>[4x]MNAHSKEMAPLMGKRTTAPGGNPVVLTEKRPADLTPTKKSAHFFLEIEGFEPNPTVTKTSPPIFSKPMDSNIRQCLSGNCDDMDSPQSPQDDVTETPSNPNSPSANLAKEEQRQKKKRLKKRIFAAVSEGCVEELRELLQDLQDLCRRRRGLDVPDFLMHKLTASDTGKTCLMKALLNINPNTKEIVRILLAFAEENDILDRFINAEYTEEAYEGQTALNIAIERRQGDITAVLIAAGADVNAHA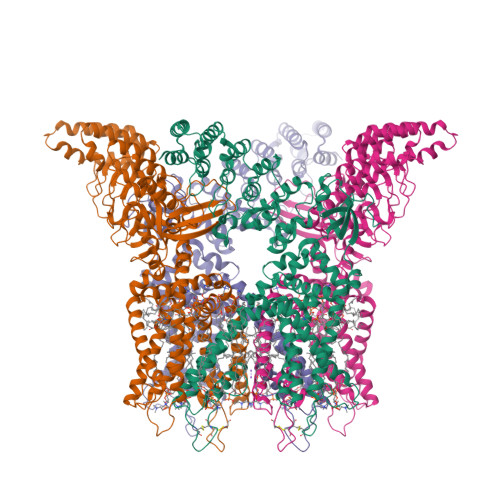KGVFFNPKYQHEGFYFGETPLALAACTNQPEIVQLLMENEQTDITSQDSRGNNILHALVTVAEDFKTQNDFVKRMYDMILLRSGNWELETMRNNDGLTPLQLAAKMGKAEILKYILSREIKEKPLRSLSRKFTDWAYGPVSSSLYDLTNVDTTTDNSVLEIIVYNTNIDNRHEMLTLEPLHTLLHTKWKKFAKYMFFLSFCFYFFYNITLTLVSYYRPREDEDLPHPLALTHKMSWLQLLGRMFVLIWATCISVKEGIAIFLLRPSDLQSILSDAWFHFVFFVQAVLVILSVFLYLFAYKEYLACLVLAMALGWANMLYYTRGFQSMGMYSVMIQKVILHDVLKFLFVYILFLLGFGVALASLIEKCSKDKKDCSSYGSFSDAVLELFKLTIGLGDLNIQQNSTYPILFLFLLITYVILTFVLLLNMLIALMGETVENVSKESERIWRLQRARTILEFEKMLPEWLRSRFRMGELCKVADEDFRLCLRINEVKWTEWKTHVSFLNEDPGPIRRTADLNKIQDSSRSNSKTTLYAFDELDEFPETSVLVPRGSAAAWSHPQFEK>MRDYSELEIFEGNPLDKWNDIIFHASKKLSKKELERLLELLALLETFIEKEDLEEKFESFAKALRIDEELQQKIESRKTDIVIQSMANILSGSGSGSGSSGNPLDKWNDIIFHASKKLSKKELERLLELLALLETFIEKEDLEEKFESFAKALRIDEE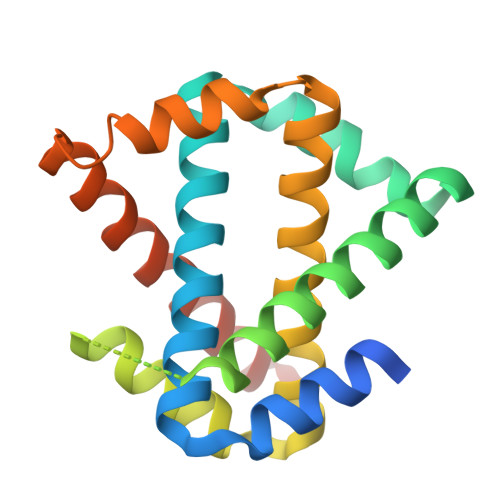LQQKIESRKTDIVIQSMANILSGLEHHHHHH[2x]> MIYYIKDLKVKGKIFENLMNKEAVEGLITFLKKAEFEIYSRENYSKYNKWFEMWKSPTSSLVFWKNYSFRCHLLFVIEKDGECLGIPASVFESVLQI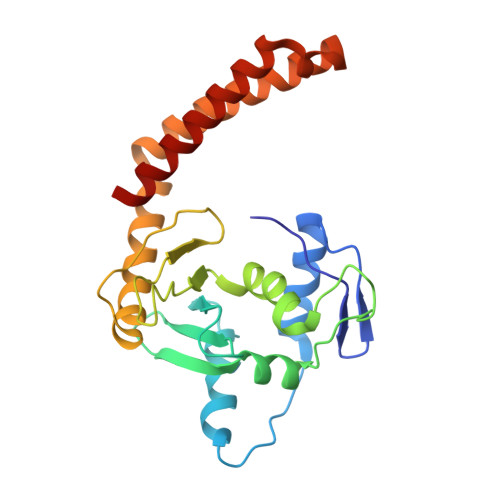YLADPFAPDTKELFVEVCNLYECLADVTVVEHFEAEESAWHKLTHNETEVSKRVYSKDDDELLKYIPEFLDTIATNKKSQKYNQIQGKIQEINKEIATLYESSEDYIFTEYVSNLYRESAKLEQHSKQILKE> LGSARRLYVGNIPFGITEEAMMDFFNAQMRLGGLTQAPGNPVLAV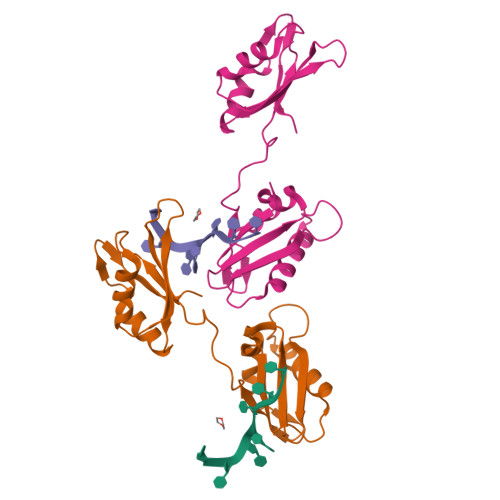QINQDKNFAFLEFRSVDETTQAMAFDGIIFQGQSLKIRRPHDYQPLPGAHKLFIGGLPNYLNDDQVKELLTSFGPLKAFNLVKDSATGLSKGYAFCEYVDINVTDQAIAGLNGMQLGDKKLLVQRAS>[9x]MTTSINSVVTVFQNVFTNHGSTLLNGILIATTVGGQSLVRKLTFSCPCAYPLNIYHSLVFMFGPTAALLLIGITVNSTTWKLAHGFFFRVRDTRHSWKTTCVSWIEVLI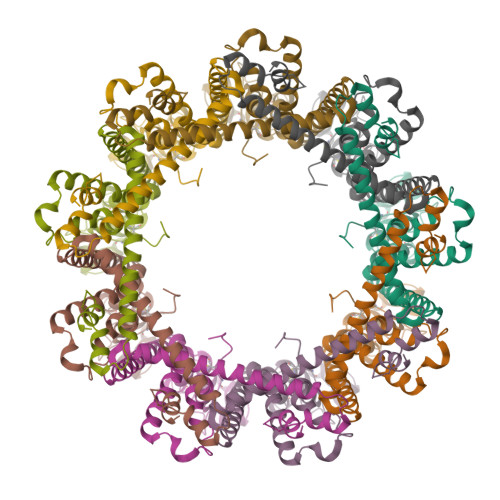QSSVAPIAWLFVVFLDGGYYRCYRSHEFCLISDAILCKNSTILNSYASTSSFNKISDNGKYCPPCICVPNPTDASYLEAESQIYAWGLLLFSGVAAFLVITCNRMCDKYTLVQRQYVETYKNVETQKFDAVAKEHASQLAEHNARAFFGQKDWTKRDWDWVSGIPEVNNPLFARLRLIAAEKTQQTMYTPLQLWNDNKGYRIPQPDLQLTQIIVDETKEDLEENLYFQ>MWKDKEFQVLFVLTILTLISGTIFYSTVEGLRPIDALYFSVVTLTTVGSELMPQTDFGKIFTILYIFIGIGLVFGFIHKLAVNV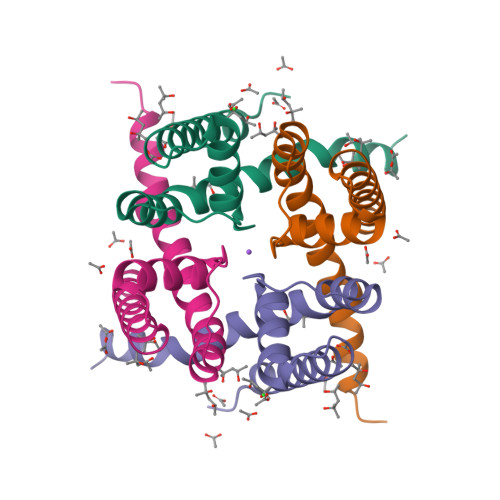QLPSILSNLVPR[2x]>[2x]MNHKVHHHHHHMKANQVQPLNKYPVVFVHGFLGLVGDNAPALYPNYWGGNKFKVIEELRKQGYNVHQASVSAFGSNYDRAVQLYYYIKGGRVDYGAAHAAKYGHERYGKTYKGIMPNWEPGKKVHLVGHAMGGQTIRLMEEFLRNGNKEEIAYHQAHGGEISPLFTGGHNNMVASITTLATPHNGSQAADKFGNTEAVRKIMFALNRFMGNKYSNIDLGLTQWGFKQLPNESYIDYIKRVSKSKIWTSDDNAAYDLTLDGSAKLNNMTSMNPNITYTTYTGVSSHTGPLGYENPDLGTFFLMDTTSRIIGHDAREEWRKNDGVVPVISSLHPSNQPFVNVTNNEPATRRGIWQVKPILQGWDHVDFIGVDFLDFKRKGSELANFYIGIINDLLSVEATEGKGTQLKAS

SA lipase (SAL, also known as glycerol ester hydrolase), a triacylglycerol esterase, shows strong cytopathic activity in host cells. SAL, an ester bond-hydrolyzing enzyme, is secreted in prepolypeptide form containing 690 amino acid residues and is processed into its mature form containing 394 amino acid residues. Its active site is composed of a typical catalytic triad including Ser116, Asp 307, and His349 residues, similar to other serine hydrolases. The SAL crystal structure exhibited a typical α/β-hydrolase fold comprising a central twisted β-sheet flanked by α-helices on both sides.

An inactive Ser116 mutant with Ala substitution, which lost PNPB-hydrolyzing activity, was also constructed. The SAL–orlistat complex, which was isomorphous with native SAL, showed strong positive electron density maps of orlistat molecules near the active sites of chains A and B. The crystallization condition of the S116A mutant crystal was different than the native SAL crystal, with the former displaying a hexagonal system and with two molecules in the asymmetric unit. The S116A mutant crystal had a different crystallization condition than the native crystal, as shown by the distinct dimeric form. The S116A mutant crystal structure also bound to fatty acids near the Ser116 residue. Wild-type S116A and S116A mutant differentially bound to fatty acids at the active site due to amino acid differences between Ser and Ala. The carboxylate moieties of fatty acids shifted closer to Ala116 in the mutant than in the wild type. In the native SAL crystal, three fatty acids were observed near the active site, whereas only one fragment was bound to S116A mutant. The fatty acid bound in the S116A mutant was located on the short α-side chain and was almost 12 carbon atoms in length. The native and S116A mutant crystals did not use PEG under the crystallization condition or during cultivation or purification.> MENFTTNLNQLARVGGIDPLIGREKELERAIQVLCRRRKNNPLLVGESGVGKTAIAEGLAWRIVQGDVPEVMADCTIYSLDIGS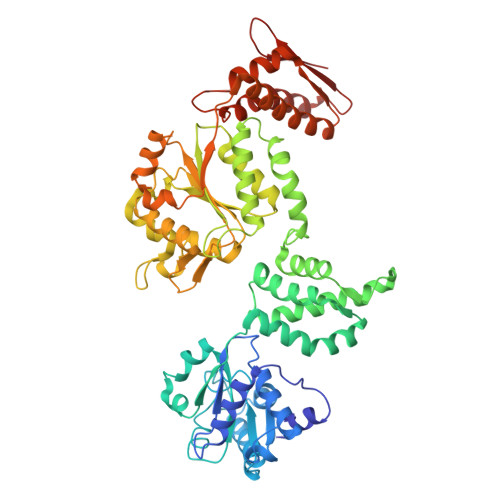LLAGTKYRGDFEKRFKALLKQLEQDTNSILFIDEIHTIIGAGAASGGQVDAANLIKPLLSSGKIRVIGSTTYQEFSNIFEKDRALARRFQKIDITEPSIEETVQIINGLKPKYEAHHDVRYTAKAVRAAVELAVKYINDRHLPDKAIDVIDEAGARARLMPVSKRKKTVNVADIESVVARIARIPEKSVSQSDRDTLKNLGDRLKMLVFGQDKAIEALTEAIKMARAGLGHEHKPVGSFLFAGPTGVGKTEVTVQLSKALGIELLRFDMSEYMERHTVSRLIGAPPGYVGFDQGGLLTDAVIKHPHAVLLLDEIEKAHPDVFNILLQVMDNGTLTDNNGRKADFRNVVLVMTTNAGVRETERKSIGLIHQDNSTDAMEEIKKIFTPEFRNRLDNIIWFDHLSTDVIHQVVDKFIVELQVQLDQKGVSLEVSQEARNWLAEKGYDRAMGARPMARVIQDNLKKPLANELLFGSLVDGGQVTVALDKEKNELTYGF>GAMRKIGIIGGTFDPPHYGHLLIANEVYHALNLEEVWFLPNQIPPHKQGRNITSVESRLQMLELATEAEEHFSICLEELSRKGPSYTYDTMLQLTKKYPDVQFHFIIGGDMVEYLPKWYNIEALLDLVTFVGVARPGYKLRTPYPITTVEIPEFAVSSSLL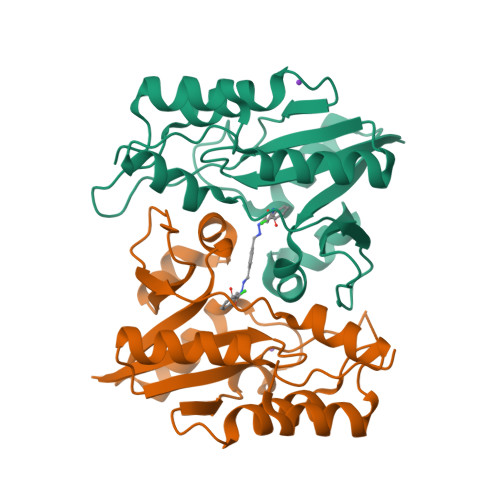RERYKEKKTCKYLLPEKVQVYIERNGLYES[2x]>[4x]SNAMEKTVGNAVKGGSFLVDEITIDQVFTPEDFSSEHKMIAKTTEDFIVNEVLPELEYLEQHEFDRSVRLLKEAGELGLLGADVPEEYGGIGLDKVSSALIAEKFSRAGGFAITHGAHVGIGSLPIVLFGNEEQKKKYLPLLATGEKLAAYALTEPGSGSDALGAKTTARLNAEGTHYVLNGEKQWITNSAFADVFIVYAKIDGEHFSAFIVEKDYAGVSTSPEEKKMGIKCSSTRTLILEDALVPKENLLGEIGKGHIIAFNILNIGRYKLGVGTVGSAKRAVEISAQYANQRQQFKQPIARFPLIQEKLANMAAKTYAAESSVYRTVGLF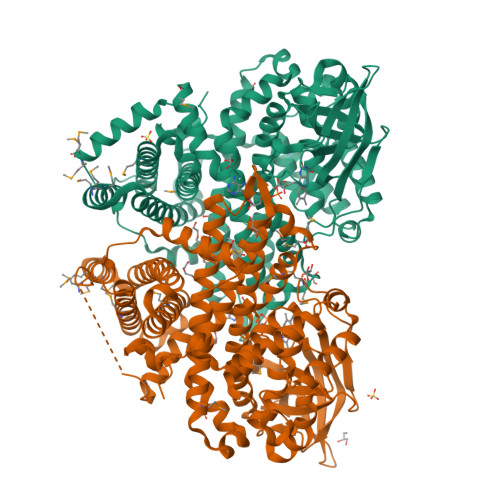ESRMSTLSEEEVKDGKAVAASIAEYAIECSLNKVFGSEVLDYTVDEGVQIHGGYGFMAEYEIERMYRDSRINRIFEGTNEINRLIVPGTFLRKAMKGELPLLQKAQKLQEELMMMMPEEVGDEPLALQKYLVNNAKKIGLMVAGLAAQKYGKALDKEQEILVNIADIVSNLYAMESAVLRTEKAIKTTGLEKNKQKVLYTEVFCQEAFNEIEAHAKETLIAVENGDMLRMMLSSLRKLTRHTPLNVIPKKREIAAKILEDERYTV> LPTSNPAQELEARQLERTTRDDLINGNSASCADVIFIYARGSTETGNLGTLGPSIASNLESAFGKDGVWIQGVGGAYRAPLGDNALPRGTSSAA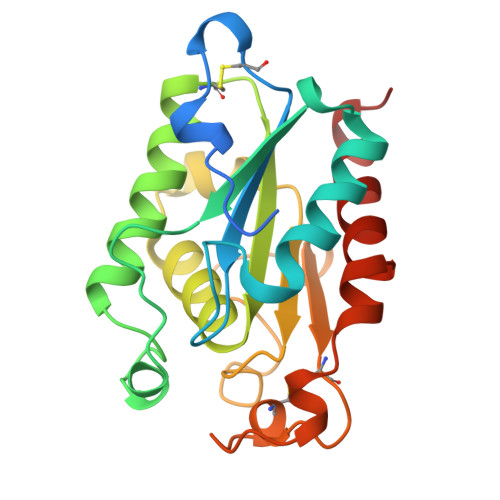IREMLGLFQQANTKCPDATLIAGGYSQGAALAAASIEDLDSAIRDKIAGTVLFGYTKNLQNRGRIPNYPADRTKVFCNTGDLVCTGSLIVAAPHLAYGPDARGPAPEFLIEKVRAVRGSA>GRKKIQITRIMDERNRQVTFTKRKFGLMKKAYELSVLCDCEIALIIFNSSNKLFQYASTDMDKVLLKYTEYNEPHESRTNSDIVEALNKK[6x];> HMSPGDSRRLSIQRCIQSLVHACQCRNANCSLPSCQKMKRVVQH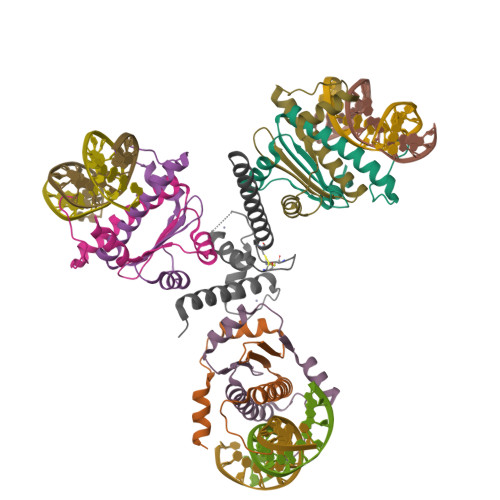TKGCKRKTNGGCPICKQLIALCCYHAKHCQENKCPVPFCLNIKQKLRQQQLQHRLQQAQMLRRRMASM>[3x]PTLEVFLPAGHDDARKAELIARLTGATVDSIGAPIESVRVLLTELPATHIGLGGRSAADGAPPSLPVIVAILIAGRTDEQKRALIAALSETSASVLDAPLQATRVMIKDIPNTDFGIGGQTARALGR

Here, we have described a global mapping of structure–function relationships among the members of the tautomerase superfamily (TSF)4 (3, 4). From a structural perspective, the functionally diverse members of the TSF share a small, structurally similar core domain that comprises a β-α-β motif. All biochemically characterized enzymes in the superfamily fall into five reaction types, each of which uses the N-terminal proline either as a general base or a general acid. The domain structure of the TSF is relatively simple, with nearly all of the members represented by either a single β-α-β structural motif or as fusion proteins composed of two of these subdomains.

Starting from the short 4-OT, the transition to the Fused 4-OT reflects the fusion of the single β-α-β unit represented by the short 4-OTs to form proteins with two β-α-β subdomains that are roughly twice as long as the short 4-OTs. The percent identity for each pair of sequences along the similarity path is 42% between 4-OT and the Fused 4-OT, 41% between Fused 4-OT and Linker 2, 26% between Linker 2 and Linker 1, 31% between Linker 1 and CgX, and 33% between CgX and cis-CaaD. Among the characterized fusion proteins of the TSF, only two enzymes showed substantial 4-OT activity, Fused 4-OT and Linker 2. CHMI has been reported to have 4-OT activity as well. Fig. S6 indicates that the characterized Fused 4-OT protein matches best with 4-OT Level 2 subgroup 1. Indeed, both Fused 4-OT and Linker 2 were shown to be proficient tautomerases with 2-HM, whereas Linker 1, cis-CaaD, and CgX showed no activity. Compared with 4-OT, Linker 2 exhibited only a 2-fold drop in kcat/Km, whereas Fused 4-OT showed a 23-fold drop in kcat/Km. Linker 1 and Fused 4-OT do not show cis-CaaD activity. Especially interesting is that two of the key structural connections linking the 4-OT and cis-CaaD subgroups, Fused 4-OT and Linker 2, also exhibit multiple links to the MIF and MSAD subgroups as well as links between the cis-CaaD subgroup and the MIF and MSAD subgroups. We speculate that the central position of Fused 4-OT and Linker 2 in the structure similarity network offers a starting point for new studies aimed at addressing the evolution of the contemporary TSF subgroups from an ancient scaffold.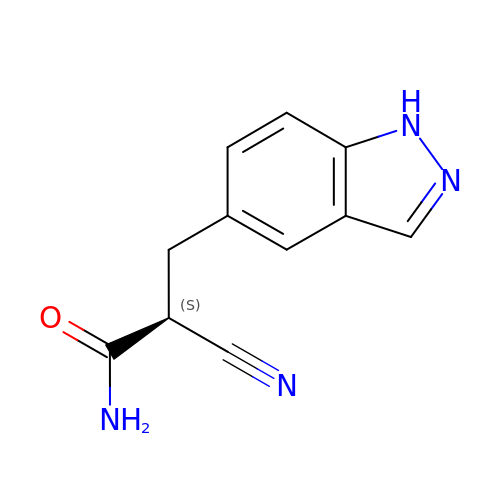(2S)-2-cyano-3-(1H-indazol-5-yl)propanamide | C11 H10 N4 O | LSZLZUAHIJIGOY-QMMMGPOBSA-N> AEIGGDHGYNATNIAAGQTSGAVTQIGPAVMGMV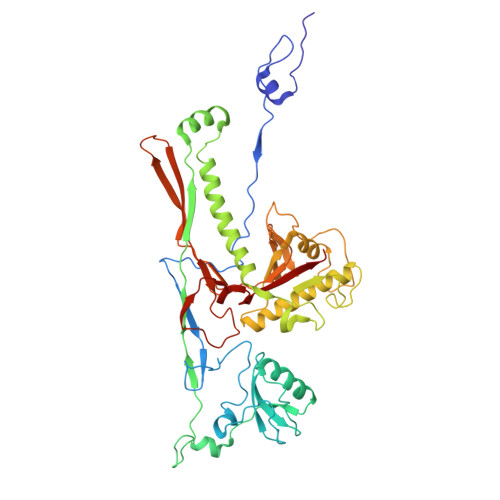RRAIPNLIAFDICGVQPMNSPTGQVFALRAVYGKDPVAAGAKEAFHPMYGPDAMFSGQGAAKKFPALAASTQTTVGDIYTHFFQETGTVYLQASVQVTIDAGATDAAKLDAEIKKQMEAGALVEIAEGMATSIAELQEGFNGSTDNPWNEMGFRIDKQVIEAKSRQLKAAYSIELTQDLRAVHGMDADAELSGILATEIMLEINREVVDWINYSAQVGKSGMTLTPGSKAGVFDFQDPIDIRGARWAGESFKALLFQIDKEAVEIARQTGRGEGNFIIASRNVVNVLASVDTGISYAAQGLATGFSTDTTKSVFAGVLGGKYRVYIDQYAKQDYFTVGYKGPNEMDAGIYYAPYVALTPLRGSDPKNFQPVMGFKTRYGIGINPFAESAAQAPASRIQSGMPSILNSLGKNAYFRRVYVKGI> KKISNPIIPY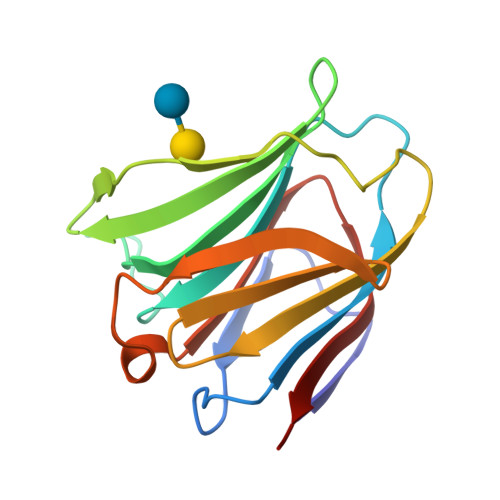VGTILGGLVPGELIVLHGSIPDDADRFQVDLQCGSSIKPRADVAFHFNPRFKWSGCVVCNTLEREKWGWEEITYEMPFQKGRPFEIVIMILKDKFQVSVNKKHLLLYNHRISLERIDTLGIYGKVQIKSIEFVSN>MKELIRKLTEAFGPSGREEEVRSIILEELEGHIDGHRIDGLGNLIVWKGSGEKKVILDAHIDEIGVVVTNVDDKGFLTIEPVGGVSPYMLLGKRIRFENGTIGVVGMEGETTEERQENVRKLSFDKLFIDIGANSREEAQKMCPIGSFGVYDSGFVEVSGKYVSKAMDDRIGCAVIVEVFKRIKPAVTLYGVFSVQEEVGLVGASVAGYGVPADEAIAIDVTDSADTPKAIKRHAMRLSGGPALKVKDRASISSKRILENLIEIAEKFDIKYQMEVLTFGGTNAMGYQRTREGIPSATV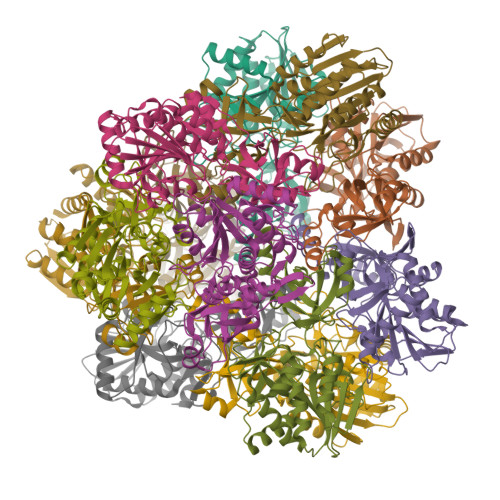SIPTRYVHSPSEMIAPDDVEATVDLLIRYLGA[12x]> VTNVGEDGEPGETEPRHALSPVDMHVHTDVSFLLDRFFDVETLELSNLTGSPATHVLDPFGSTAQLAWARLLNTCTYFFSDLELSIQFKFTTTPSSVGEGFVWVKWFPVGAPTKTTDA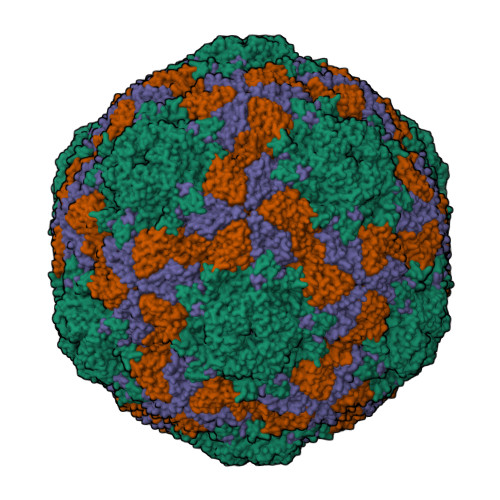WQLEGGGNSVRIQQLAVAGMSPTVVFKIAGSRSQACGFSVPYTSMWRVVPVFYNGWGAPTKEKATYNWLPGAHFGSILLTSDAHDKGGCYLRYRFPRANMYCPRPIPPAFTRPADKTRHKFPTNINKQ;> DKKTEETTNIEDRIETTVVGVTIINSQGSVGTTYCYSKPDGRPPSTVSDPVTRLGPTLSRHYTFKVGEWPHSQSHGHAWICPLPSDKLKKMGSFHEVVKAHHLVKNGWDVVVQVNASFAHSGALCVAAVPEYEHTHEKALKWSELEEPAYTYQQLSVFPHQLLNLRTNSSVHLVMPYIGPGPTTNLTLHNPWTIVILILSELTGPGQTVPVTMSVAPIDAMVNGPLPNPE;> APIRVVSVPESDSFMSSVPDNSTPLYPKVVVPPRQVPGRFTNFIDVAKQTYSFCSISGKPYFEVTNTSGDEPLFQMDVSLSAAELHGTYVASLSSFFAQYRGSLNFNFIFTGAAATKAKFLVAFVPPHSAAPKTRDEAMACIHAVWDVGLNSAFSFNVPYSSPADFMAVYSAEATVVNVSGWLQVYALTALTSTDIAVNSKGRVLVAVSAGPDFSLRHPVDLPDKQ;> GAGTSTPTTGNQNMSGNSGSIVQNFYMQQYQNSIDADLGDNVISPEGQGSNTSSSTSSSQSSGLGGWFSSLLNLGTKLLA In this work, we describe the rational design, production, and characterization of K1K1, a novel minimal MET agonist consisting of two copies of the kringle 1 domain of HGF/SF in tandem orientation. On the strength of the structural, biochemical, and mutagenesis data available, we rationalized that a covalent dimer containing a tandem repeat of the K1 domain of HGF/SF could constitute a minimal and stable MET agonist able to diffuse effectively across tissue boundaries owing to the absence of the N-terminal domain of HGF/SF responsible for high-affinity binding to heparan sulphate proteoglycans (HSPG). Therefore, we designed a linker to bridge the distance between the C-terminus of the first K1 domain and the N-terminus of the second one. We chose for that purpose the four–amino acid long linker, SEVE, which is naturally present between kringle 1 and kringle 2 (K2) in HGF/SF.

The collected datasets enabled the determination of the molecular structures at 1.8 Å resolution and 1.7 Å for K1K1 and K1K1H6, respectively. Both proteins crystalized in space group P 1 21 1 with K1K1 having two molecules per asymmetric unit and K1K1H6 having one. Structurally, K1K1 and K1K1H6 are nearly identical with a backbone root mean square deviation of 0.8 or 1.8 Å, depending on which of the two molecules in the asymmetric unit of K1K1 is used for alignment with K1K1H6. Both proteins show an elongated “stretched-out” conformation with the MET-binding sites exposed on opposite ends and the N- and C-terminus located at the centre. Surprisingly, like the revelation of seeing the first structures of NK1 that presented a likely biologically relevant dimer, both crystal structures show a pseudo C2 symmetry around a central axis and present both receptor-binding sites in nearly identical orientation on either side of the molecule (located around residue Glu37 in the first kringle and residues Glu120 in the second kringle, equivalent to NK1 residue Glu159). One can envision a binding mode in which two MET receptor monomers are brought in proximity by binding on opposite sides of K1K1, forming a 2:1 receptor activation complex. Alignment of the first kringle domain of K1K1 with one of the two kringle domains within the NK1 dimer places the second K1K1 kringle close to the position of the kringle domain of NK1 protomer 2. However, the straightened conformation observed in the crystal structure of K1K1 “misaligns” the second K1K1 kringle domain through a rotation by 109.7 degrees and a translation of roughly 14 Å. No contacts between the two K1 domains or the kringle domains with the SEVE linker are observed. The linker is more stretched out compared with the two NK2 structures supporting our idea that it is highly flexible and therefore allows significant conformational freedom. This flexibility was confirmed with SAXS measurements of K1K1 in solution which generated an envelope that perfectly accommodates K1K1 volume-wise but only in a bent conformation.

>[2x]AIRNCIIGKGRSYKGTVSITKSGIKCQPWSSMIPHEHSFLPSSYRGKDLQENYCRNPRGEEGGPWCFTSNPEVRYEVCDIPQCSEVECIIGKGRSYKGTVSITKSGIKCQPWSSMIPHEHSFLPSSYRGKDLQENYCRNPRGEEGGPWCFTSNPEVRYEVCDIPQCSEVE>[4x]MSQPRTVTVLGATGSIGHSTLDLIERNLDRYQVIALTANRNVKDLADAAKRTNAKRAVIADPSLYNDLKEALAGSSVEAAAGADALVEAAMMGADWTMAAIIGCAGLKATLAAIRKGKTVALANKESLVSAGGLMIDAVREHGTTLLPVDSEHNAIFQCFPHHNRDYVRRIIITASGGPFRTTSLAEMATVTPERAVQHPNWSMGAKISIDSATMMNKGLELIEAFHLFQIPLEKFEILV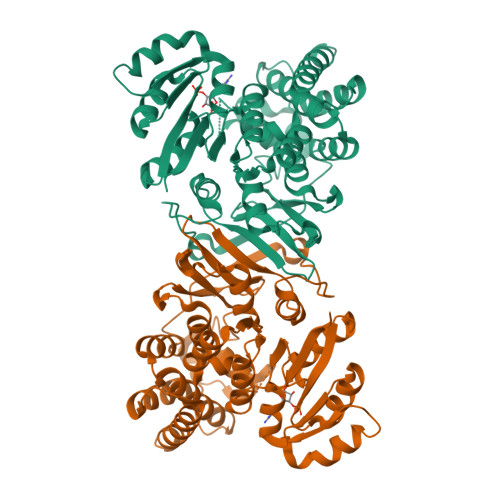HPQSVIHSMVEYLDGSILAQIGSPDMRTPIGHTLAWPKRMETPAESLDFTKLRQMDFEAPDYERFPALTLAMESIKSGGARPAVMNAANEIAVAAFLDKKIGFLDIAKIVEKTLDHYTPATPSSLEDVFAIDNEARIQAAALMESLPA>MGLQTVMKWKTVVAIFVVVVVYLVTGGLVFRALEQPFESSQKNTIALEKAEFLRDHVCVSPQELETLIQHALDADNAGVSPIGNSSNNSSHWDLGSAFFFAGTVITTIGYGNIAPSTEGGKIFCILYAIFGIPLFGFLLAGIGDQLGTIFGKSIARV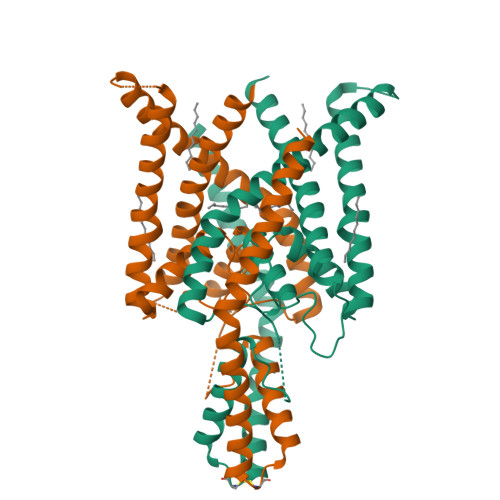EKVFRKKQVSQTKIRVISTILFILAGCIVFVTIPAVIFKYIEGWTALESIYFVVVTLTTVGFGDFVAGGNAGINYREWYKPLVWFWILVGLAYFAAVLSMIGDWLRVLSKKTKEEVGEAENLYFQ[4x]>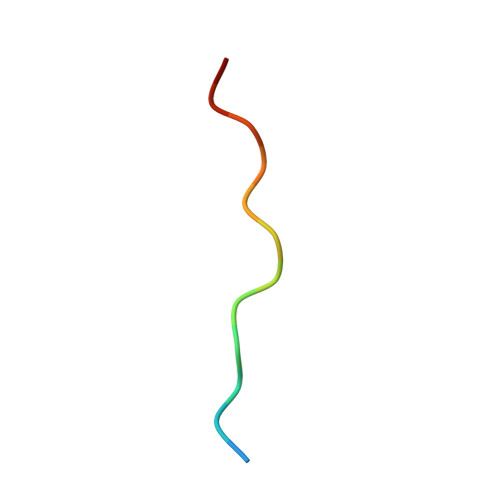 XQTPTLGPIQPTRX> QDWLTFQKKHITNTRDVDCDNIMSTNLFHCKDKNTFIYSRPEPVKAICKGIIASKNVLTTSEFYLSDCNVTSRPCKYKLKKSTNKFCVTCENQAPVHFVGVGSC

Onconase® (ONC, Alfacell Corporation, Somerset, NJ, USA) is a ribonuclease with anti-tumor activity isolated from oocytes of the Northern leopard frog, Rana pipiens. ONC is a member of the pancreatic ribonuclease superfamily whose archetypal member, ribonuclease A (RNase A; EC 3.1.27.5), holds a central position in the study of protein chemistry, enzymology and molecular evolution. Although ONC has only 30% sequence identity with RNase A, contains 20 fewer residues (104 versus 124) and possesses an alternative disulfide bonding arrangement, it has a highly similar α/β fold. The ribonucleolytic activity of ONC is essential to its cytotoxicity, and the target of this activity is intracellular RNA.

Redressing this, we have determined the X-ray crystal structure of ONC at atomic resolution. The atomic resolution structure of ONC·SO4 was determined from an orthorhombic crystal at 100 K. The data also enabled the resolution of discrete alternate conformations for the side chains of six residues (Asp18, Ile51, Ser54, Thr60, Thr83 and Asn84) to the extent that their 2Fo−Fc electron density is continuous when contoured at up to 1.4 σ. Hence, at the P1 subsite, residues Lys9, His10, His97 (the latter in the inactive, B conformation) and Phe98 (the counterparts of RNase A residues Gln11, His12, His119 and Phe120, respectively) coordinate a sulfate ion. The N-terminal pyroglutamate residue (Pca1), which serves to align Lys9 for catalysis, is now refined in a puckered conformation rather than the planar one described by the rtONC·SO4 coordinates. The refinement directs its side chain into a more extended conformation than that reported for rtONC·SO4, placing the Nζ atom 5.22 Å from the nearest sulfate O atom (cf. 5.37 Å in rtONC·SO4). This leaves it within hydrogen-bonding range of the O atom of Lys33 (2.92 Å distant) and the Oδ1 atom of Asn34 (3.03 Å distant), although it should be noted that electron density for Lys31 is lacking beyond Cδ, indicating that the side chain of this residue has significant mobility and most likely makes no firm hydrogen bonds in the presence of sulfate. The side chain of this residue is partially disordered with weak electron density beyond Cβ, and the refinement suggests that the major side chain rotamer intrudes into the space occupied by the bound pyrimidine. Comparison with the rtONC·SO4 data reveals that the low temperature used during X-ray diffraction brings about a 7.7% compaction in unit cell volume, with the largest reduction (5.8%) affecting the b axis. This is coincident with a compaction of the protein structure, as judged by a 2.0% reduction in solvent-excluded volume (from 13685 to 13409 Å3) and a 1.0% reduction in radius of gyration (from 13.736 to 13.603 Å). Furthermore, it indicates that a significant contribution to the compaction is made by the movement of lobes 1 and 2 towards one another. Our analyses of the present structure have, for the first time, identified appreciable collective motion in ONC.> MGSSHHHHHSSGLVPRGSHMRYSLRQDIAVEPVIAGWYGWSYLLPPQTLARFVHNRFNRIVESYLDDPQVHAAAVRQRRMHGGPWIHAHEHRDAIEAWYRETAPRRERLDELFEAVRRLEEDILPRHHGECLDPVYQELPAALAGRVEVFYGRDNRTADYRFVEPLMYASEYYDESWQQVRFRPVTEDAREFALTTPMLEYGPEQLLVNVPLNSPLLDAVFRGGLTGTELDDLAARFGLDGERAARFASYFEPTPAASEAPAPASSSEEDVLEYVGHACVFARHRGTTFLVDPVLSYSGYPGGAENRFTFADLPERIDHLLITHNHQDHMLFETLLRIRHRVGRVLVPKSTNASLVDPGLGGILRRLGFTDVVEVDDLETLSCGSAEVVALPFLGEHGDLRIRSKTGWLIRFGERSVLFAADSTNISPTMYTKVAEVIGPVDTVFIGMESIGAAASWIY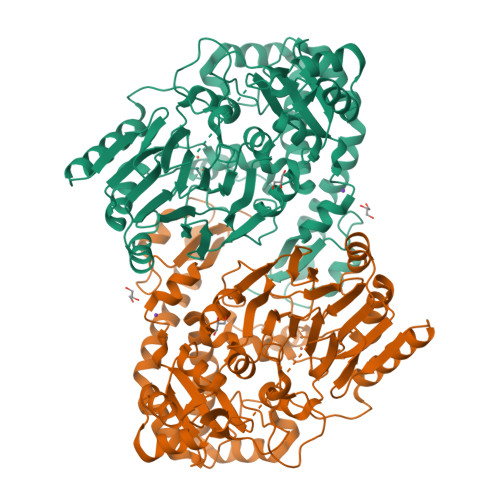GPLYGEPLDRRTDQSRRLNGSNFPQAREIVDALEPDEVYVYAMGLEPWMGVVMAVDYDESHPAIVDSDLLVRHVQDKGGTAERLHLRRTLRL> MHHHHHHSSGRENLYFQGSGTIYGWGHNHRGQLGGIEGAKVKVPTPCEALATLRPVQLIGGEQTLFAVTADGKLYATGYGAGGRLGIGGTESVSTPTLLESIQHVFIKKVAVNSGGKHCLALSSEGEVYSWGEAEDGKLGHGNRSPCDRPRVIESLRGIEVVDVAAGGAHSACVTAAGDLYTWGKGRYGRLGHSDSEDQLKPKLVEALQGHRVVDIACGSGDAQTLCLTDDDTVWSWGDGDYGKLGRGGSDGCKVPMKIDSLTGLGVVKVECGSQFSVALTKSGAVYTWGKGDYHRLGHGSDDHVRR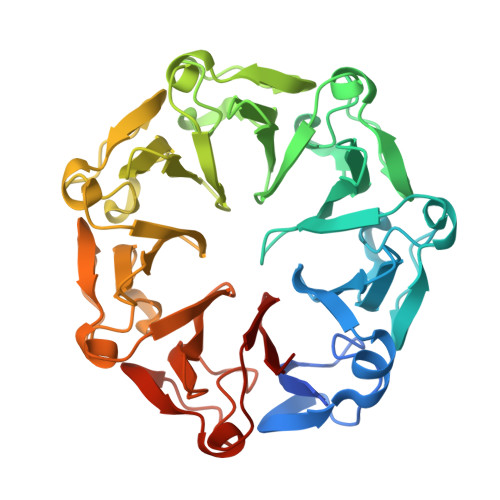PRQVQGLQGKKVIAIATGSLHCVCCTEDGEVYTWGDNDEGQLGDGTTNAIQRPRLVAALQGKKVNRVACGSAHTLAWSTSKP>MGNKNTPLNSGKHPDLKIEVAIIGAGTSGLYTAYRLVTDKKFKAHDVQIFDMNNKLGGRLESVIMPGMNFWGELGGMRYLTSQQIVTTLIEGYPLSEKDPNKRTPVLKDKMTPVPFPMGDPSKLLMYLRKERFKQNAWNEAQKKGEKLPTRYYLNENDLGFSSDQLFNKIIYDVLMADPWVAETYGSKIIKGSSVYDYSFKLTSRDWDDIKPKLVYNFPNSPYDQRKVNDIGFWNLIKDQVSQEGYEFLANAGGYYSNTINWNSAEAFPYMVGDFSAGTIYKTIEEGYDSIAYAVANSYMEHEGACIWSENKLLTFTKDHPLTNTHKYELTFLNLKTNTQWKVYANSIVLAMP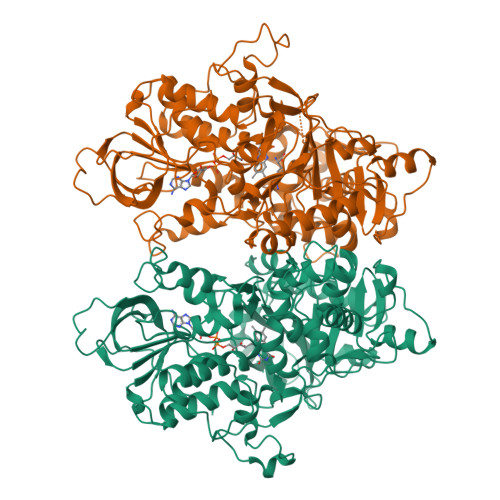RKSLELLDQNNFFFNINKNSVLNNNIRSVIMEPAFAILMGFEYPWWKELGIDSGHSITDLPMRQCYYFGTDPETNNSMLLGSYGDMETETFWKALSDDKVLFEVKAAKSASLRELHQLDDVQATKLMVGELMNQLRELHGDTVTIPEPYVTYFKDWTDEPFGAGYHAWKAGFSVENVMPYMRKPLTDEQIHICGEAYSDQQGWVEGAFCEAEKMLQEYFGLDRPYWLSPDYYLGWEHHHHHH[2x]>MHHHHHHSLLTEVETYVLSIVPSGPLKAEIAQRLEDVFAGKNTDLEVLMEWLKTRPILSPLTKGILGFVFTLTVPSERGLQRRRFVQNALNGNRDPNNMDKAVKLYSKLKSEITFHGAKEIALSYSAGALASCMGLIYNRMGAVTTEVAFG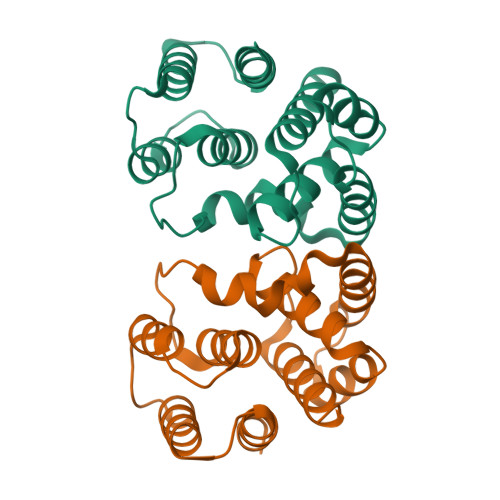LVCATCEQIADSQHRSHRQM[4x]N-[(2Z)-3,7-dimethylocta-2,6-dien-1-yl]-N'-[(1R,3S,5R,7R)-tricyclo[3.3.1.1~3,7~]dec-2-yl]ethane-1,2-diamine | C22 H38 N2 | 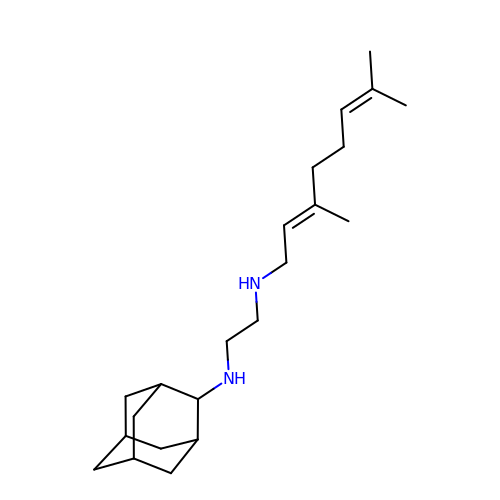JFIBVDBTCDTBRH-MDXVBTBDSA-N> MAQILPIRFQEHLQLQNLGINPANIGFSTLTMESDKFICIREKVGEQAQVVIIDMNDPSNPIRRPISADSAIMNPASKVIALKAGKTLQIFNIEMKSKMKAHTMTDDVTFWKWISLNTVALVTDNAVYHWSMEGESQPVKMFDRHSSLAGCQIINYRTDAKQKWLLLTGISAQQNRVVGAMQLYS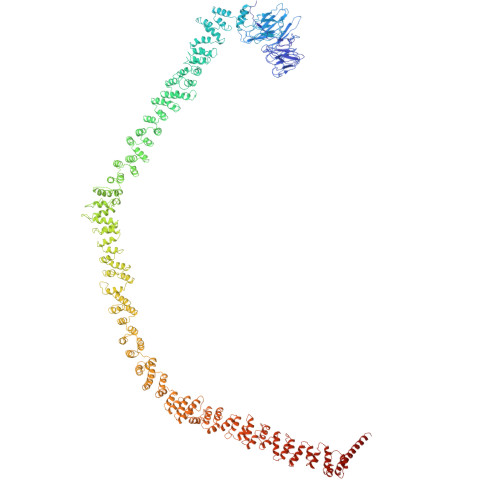VDRKVSQPIEGHAASFAQFKMEGNAEESTLFCFAVRGQAGGKLHIIEVGTPPTGNQPFPKKAVDVFFPPEAQNDFPVAMQISEKHDVVFLITKYGYIHLYDLETGTCIYMNRISGETIFVTAPHEATAGIIGVNRKGQVLSVCVEEENIIPYITNVLQNPDLALRMAVRNNLAGAEELFARKFNALFAQGNYSEAAKVAANAPKGILRTPDTIRRFQSVPAQPGQTSPLLQYFGILLDQGQLNKYESLELCRPVLQQGRKQLLEKWLKEDKLECSEELGDLVKSVDPTLALSVYLRANVPNKVIQCFAETGQVQKIVLYAKKVGYTPDWIFLLRNVMRISPDQGQQFAQMLVQDEEPLADITQIVDVFMEYNLIQQCTAFLLDALKNNRPSEGPLQTRLLEMNLMHAPQVADAILGNQMFTHYDRAHIAQLCEKAGLLQRALEHFTDLYDIKRAVVHTHLLNPEWLVNYFGSLSVEDSLECLRAMLSANIRQNLQICVQVASKYHEQLSTQSLIELFESFKSFEGLFYFLGSIVNFSQDPDVHFKYIQAACKTGQIKEVERICRESNCYDPERVKNFLKEAKLTDQLPLIIVCDRFDFVHDLVLYLYRNNLQKYIEIYVQKVNPSRLPVVIGGLLDVDCSEDVIKNLILVVRGQFSTDELVAEVEKRNRLKLLLPWLEARIHEGCEEPATHNALAKIYIDSNNNPERFLRENPYYDSRVVGKYCEKRDPHLACVAYERGQCDLELINVCNENSLFKSLSRYLVRRKDPELWGSVLLESNPYRRPLIDQVVQTALSETQDPEEVSVTVKAFMTADLPNELIELLEKIVLDNSVFSEHRNLQNLLILTAIKADRTRVMEYINRLDNYDAPDIANIAISNELFEEAFAIFRKFDVNTSAVQVLIEHIGNLDRAYEFAERCNEPAVWSQLAKAQLQKGMVKEAIDSYIKADDPSSYMEVVQAANTSGNWEELVKYLQMARKKARESYVETELIFALAKTNRLAELEEFINGPNNAHIQQVGDRCYDEKMYDAAKLLYNNVSNFGRLASTLVHLGEYQAAVDGARKANSTRTWKEVCFACVDGKEFRLAQMCGLHIVVHADELEELINYYQDRGYFEELITMLEAALGLERAHMGMFTELAILYSKFKPQKMREHLELFWSRVNIPKVLRAAEQAHLWAELVFLYDKYEEYDNAIITMMNHPTDAWKEGQFKDIITKVANVELYYRAIQFYLEFKPLLLNDLLMVLSPRLDHTRAVNYFSKVKQLPLVKPYLRSVQNHNNKSVNESLNNLFITEEDYQALRTSIDAYDNFDNISLAQRLEKHELIEFRRIAAYLFKGNNRWKQSVELCKKDSLYKDAMQYASESKDTELAEELLQWFLQEEKRECFGACLFTCYDLLRPDVVLETAWRHNIMDFAMPYFIQVMKEYLTKVDKLDASESLRKEEEQATETQ> MGSSHHHHHHSSGLVPRGSHMTAPGPACSDTPIAGLVELALSAPTFQQLMQRAGGRPDELTLIAPAS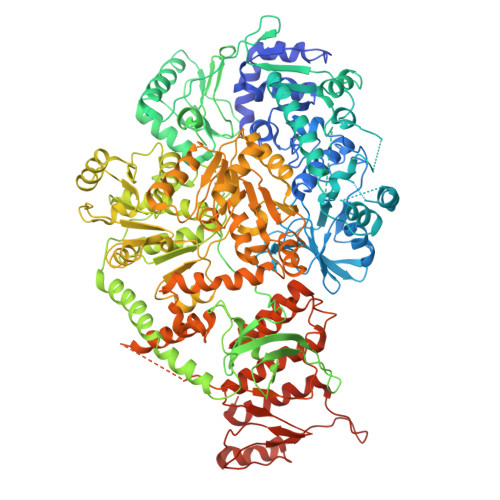ARLLVASALARQGPLLVVTATGREADDLAAELRGVFGDAVALLPSWETLPHERLSPGVDTVGTRLMALRRLAHPDDAQLGPPLGVVVTSVRSLLQPMTPQLGMMEPLTLTVGDESPFDGVVARLVELAYTRVDMVGRRGEFAVRGGILDIFAPTAEHPVRVEFWGDEITEMRMFSVADQRSIPEIDIHTLVAFACRELLLSEDVRARAAQLAARHPAAESTVTGSASDMLAKLAEGIAVDGMEAVLPVLWSDGHALLTDQLPDGTPVLVCDPEKVRTRAADLIRTGREFLEASWSVAALGTAENQAPVDVEQLGGSGFVELDQVRAAAARTGHPWWTLSQLSDESAIELDVRAAPSARGHQRDIDEIFAMLRAHIATGGYAALVAPGTGTAHRVVERLSESDTPAGMLDPGQAPKPGVVGVLQGPLRDGVIIPGANLVVITETDLTGSRVSAAEGKRLAAKRRNIVDPLALTAGDLVVHDQHGIGRFVEMVERTVGGARREYLVLEYASAKRGGGAKNTDKLYVPMDSLDQLSRYVGGQAPALSRLGGSDWANTKTKARRAVREIAGELVSLYAKRQASPGHAFSPDTPWQAELEDAFGFTETVDQLTAIEEVKADMEKPIPMDRVICGDVGYGKTEIAVRAAFKAVQDGKQVAVLVPTTLLADQHLQTFGERMSGFPVTIKGLSRFTDAAESRAVIDGLADGSVDIVIGTHRLLQTGVRWKDLGLVVVDEEQRFGVEHKEHIKSLRTHVDVLTMSATPIPRTLEMSLAGIREMSTILTPPEERYPVLTYVGPHDDKQIAAALRRELLRDGQAFYVHNRVSSIDAAAARVRELVPEARVVVAHGQMPEDLLETTVQRFWNREHDILVCTTIVETGLDISNANTLIVERADTFGLSQLHQLRGRVGRSRERGYAYFLYPPQVPLTETAYDRLATIAQNNELGAGMAVALKDLEIRGAGNVLGIEQSGHVAGVGFDLYVRLVGEALETYRDAYRAAADGQTVRTAEEPKDVRIDLPVDAHLPPDYIASDRLRLEGYRRLAAASSDREVAAVVDELTDRYGALPEPARRLAAVARLRLLCRGSGITDVTAASAATVRLSPLTLPDSAQVRLKRMYPGAHYRATTATVQVPIPRAGGLGAPRIRDVELVQMVADLITALAGKPRQHIGITNPSPPGEDGRGRNTTIKERQP> CEEPPTFEAMELIGKPKP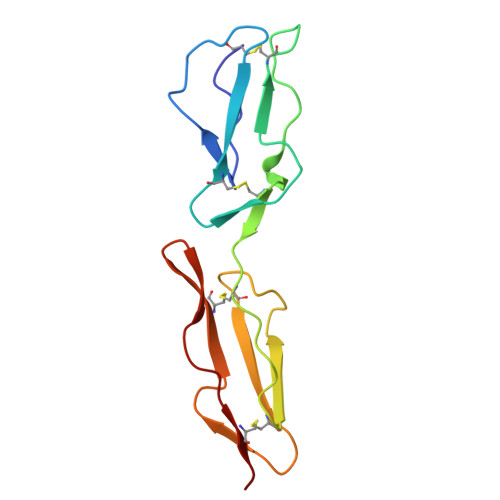YYEIGERVDYKCKKGYFYIPPLATHTICDRNHTWLPVSDDACYRETCPYIRDPLNGQAVPANGTYEFGYQMHFICNEGYYLIGEEILYCELKGSVAIWSGKPPICEKV paranitrophenyl-alpha-L-galactopyranoside | C12 H15 N O8 | 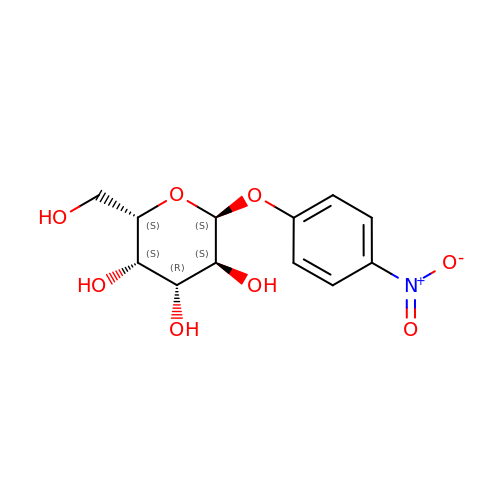IFBHRQDFSNCLOZ-MTVMDMGHSA-N gallinamide A, 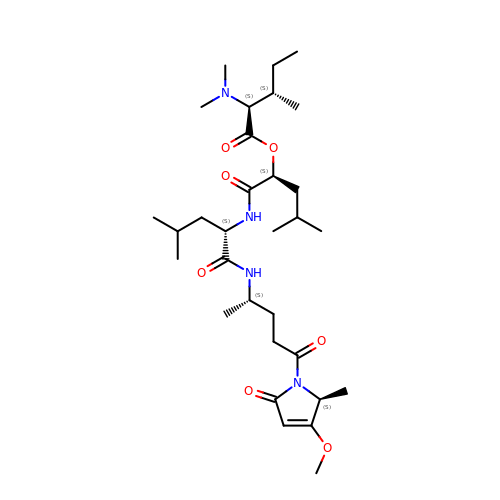bound form | C31 H54 N4 O7 | KQLKGAFEYUEPPA-ISUPFBBGSA-N>[2x]MGSSHHHHHHSQDPNSMPDNTIQWDKDADGIVTLTMDDPSGSTNVMNEAYIESMGKAVDRLVAEKDSITGVVVASAKKTFFAGGDVKTMIQARPEDAGDVFNTVETIKRQLRTLETLGKPVVAAINGAALGGGLEIALACHHRIAADVKGSQLGLPEVTLGLLPGGGGVTRTVRMFGIQNAFVSVLAQGTRFKPAKAKEIGLVDELVATVEELVPAAKAWIKEELKANPDGAGVQPWDKKGYKMPGGTPSSPGLAAILPSFPSNLRKQLKGAPMPAPRAILAAAVEGAQVDFDTASRIESRYFASLVTGQVAKNMMQAFFFDLQAINAGGSRPEGIGKTPIKRIGVLGAGMMGAGIAYVSAKAGYEVVLKDVSLEAAAKGKGYSEKLEAKALERGRTTQERSDALLARITPTADAADFKGVDFVIEAVFENQELKHKVFGEIEDIVEPNAILGSNTSTLPITGLATGVKRQEDFIGIHFFSPVDKMPLVEIIKGEKTSDEALARVFDYTLAIGKTPIVVNDSRGFFTSRVIGTFVNEALAMLGEGVEPASIEQAGSQAGYPAPPLQLSDELNLELMHKIAVATRKGVEDAGGTYQPHPAEAVVEKMIELGRSGRLKGAGFYEYADGKRSGLWPGLRETFKSGSSQPPLQDMIDRMLFAEALETQKCLDEGVLTSTADANIGSIMGIGFPPWTGGSAQFIVGYSGPAGTGKAAFVARARELAAAYGDRFLPPESLLS;>[2x]MSEEAFIYEAIRTPRGKQKNGSLHEVKPLSLVVGLIDELRKRHPDLDENLISDVILGCVSPVGDQGGDIARAAVLASGMPVTSGGVQLNRFCASGLEAVNTAAQKVRSGWDDLVLAGGVESMSRVPMGSDGGAMGLDPATNYDVMFVPQSIGADLIATIEGFSREDVDAYALRSQQKAAEAWSGGYFAKSVVPVRDQNGLLILDHDEHMRPDTTKEGLAKLKPAFEGLAALGGFDDVALQKYHWVEKINHVHTGGNSSGIVDGAALVMIGSAAAGKLQGLTPRARIVATATSGADPVIMLTGPTPATRKVLDRAGLTVDDIDLFELNEAFASVVLKFQKDLNIPDEKLNVNGGAIAMGHPLGATGAMILGTMVDELERRNARRALITLCIGGGMGVATIIERV

The Mycobacterium tuberculosis trifunctional enzyme (MtTFE) is an α2β2 tetrameric enzyme in which the α-chain harbors the 2E-enoyl-CoA hydratase (ECH) and 3S-hydroxyacyl-CoA dehydrogenase (HAD) active sites, and the β-chain provides the 3-ketoacyl-CoA thiolase (KAT) active site. Linear, medium-chain and long-chain 2E-enoyl-CoA molecules are the preferred substrates of MtTFE. Mtb is capable of switching its metabolic preference during the latent stage of infection in order to utilize host-derived fatty acids as a source of carbon rather than glucose or glycerol. The Mtb genome encodes an unusually large set of enzymes of the β-oxidation cycle; however, only a single trifunctional enzyme (MtTFE) that catalyzes three of the last four reactions in the β-oxidation cycle is present in Mtb, in contrast to other bacteria such as Escherichia coli, which has two TFEs. Here, 226 fragments were screened in a crystallographic fragment-binding study of MtTFE crystals, resulting in the structures of 16 MtTFE–fragment complexes.

The six fragments that bind in the substrate-binding pocket are B-E1, M-1, M-53, M-76, M-83 and M-109. Fragments B-E1 and M-83 form hydrogen bonds either to Serα512 or to both Serα441 and Serα512, both of which point into the catalytic site. These fragments also make weak interactions with the side chain of the catalytic Hisα462. B-E1 and M-83 interact weakly with the side chain of the catalytic cysteine Cysβ92. The R-SO2-R and R-SO2-OH moieties of B-E1 and M-83, respectively, bind at the same site, forming a hydrogen bond to the side chain of Glnβ149, as visualized in Supplementary Fig. S2 for the M-83 fragment. The five-membered ring of fragment B-E1 points away from the acyl-tail binding tunnel towards the KAT225 loop of the thiolase β-subunit (contacting the Leuβ228 side chain) and the H9A helix of the α-subunit (in particular Proα243). Leuβ228 and Proα243 line the groove between the I2 site and the K2 site. A single fragment (B-51) binds at the CoA-A(HAD/KAT) binding site (two binding events), one fragment (M-53) binds at the CoA-B(ECH2) binding site (one binding event) and five fragments (B-E1, M-1, M-49, M-53 and M-72) bind at the CoA-C(ECH/HAD) binding site (I2; 13 binding events). The distances from the ECH and HAD active sites to the I2 site are approximately 21 and 12 Å, respectively, and the corresponding distance from the KAT active site is approximately 44 Å, when considering the distances between the bridging pyrophosphate O atoms of the CoA molecules bound at these sites. The path is identified by the fragments B-E1, B-H11, M-1, M-49, M-53 and M-72, in addition to the CoA-C(ECH/HAD) molecule.>GHMAPIKVIADKGTPFADLLVPKLTASVTDGAVGVTVDAPVSVTAADGVLAAVTMVNDNGRPVAGRLSPDGLRWSTTEQLGYNRRYTLNATALGLGGAATRQLTFQTSSPAHLTMPYVMPGDGEVVGVGEPVAIRFDENIADRGAAEKAIKITTNPPVEGAFYWLNNREVRWRPEHFWKPGTAVDVAVNTYGVDLGEGMFGEDNVQTHFTIGDEVIATADDNTKILTVRVNGEVVKSMPTSMGKDSTPTANGIYIVGSRYKHIIMDSSTYGVPVNSPNGYRTDVDWATQISYSGVFVHSAPWSVGAQGHTNTSHGCLNVSPSNAQWFYDHVKRGDIVEVVNTVGGTLPGIDGLGD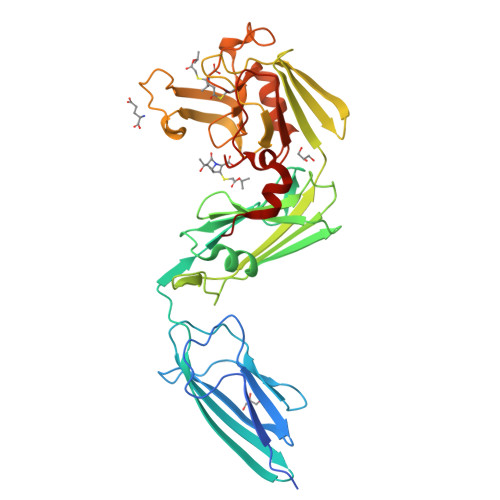WNIPWDQWRAGNAKA[2x]>[16x]GPSMHVLGEDIDASTGRFKILSLLGEGTFGKVVEAWDRKRKEYCAVKIVRNVPKYTRDAKIEIQFMERVRLSDVEDRFPLMKIQRYFQNETGHMCIVMPKYGPCLLDWIMKHGPFNHRHLAQIIFQVGAALDYFHTELHLMHTDLKPENILMESGDTSVDPMTHRALPPEP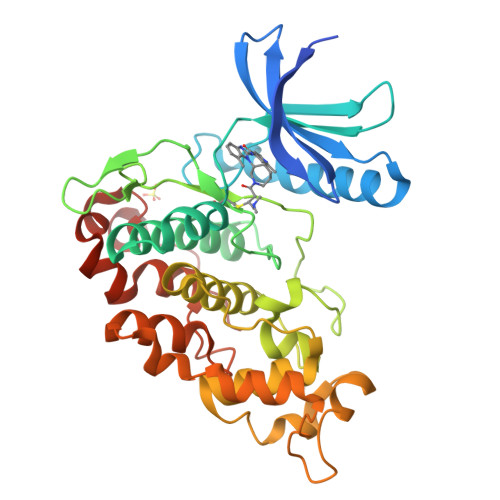CRVRICDLGGCCDERHSRTAIVSTRHYRSPEVVLSLGWMYSTDLWSMGCIIYELYTGKLLYDTHDNLEHLHLMEKTLGRLPADWSVRCGTQEARDLFTAAGTLQPCKDPKHIARIARARPVREVITEPLLCDLILNLLHYDRQRRLNARQMMSHAYVHKYFPECRQHPNHVDNRSKLPPTPVM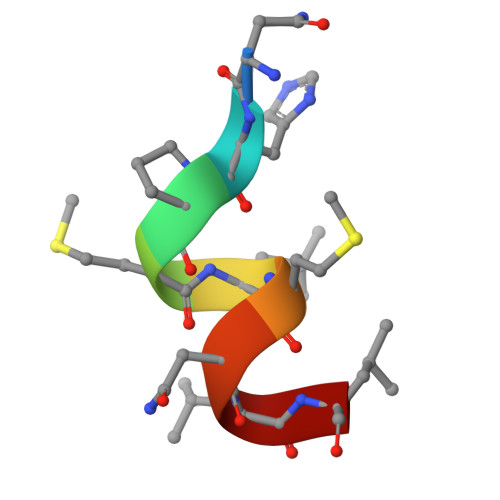> NHPMLMNLL> GSHMEAVQNRIVEAAERVPGVRGVIHLRARYVGQDIWADMIIGVDPENTVEQAEEICEAVQAA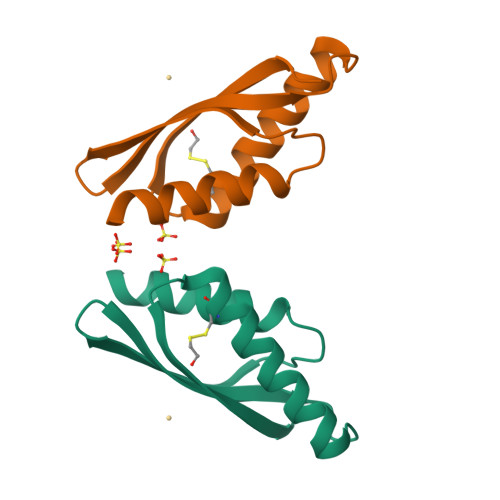VCGKIRRIESLHVSAHAREIGDTTKPSFSDQPLSFDEVMLSKVDN> MATTSHQPQDRYKAVWLIFFMLGLGTLLPWNFFMTATQYFTNRLDMSQNVSLVTAELSKDAQASAAPAAPLPERNSLSAIFNNVMTLCAMLPLLLFTYLNSFLHQRIPQSVRILGSLVAILLVFLITAILVKVQLDALPFFVITMIKIVLINSFGAILQGSLFGLAGLFPASYTAAIMSGQGLAGFFASVAMICAIASGSELSESAFGYFITACAVIILTIICYLGLPRLEFYRYYQQLKLEGPTNESHSIKAILKKISVLAFSVCFIFTITIGMFPAVTVEVKSSIAGSSTWERYFIPVSCFLTFNIFDWLGRSLTAVFMWPGKDSRWLPSLVLARLVFVPLLLLCNIKPRRYLTVVFEHDAWFIFFMAAFAFSNGYL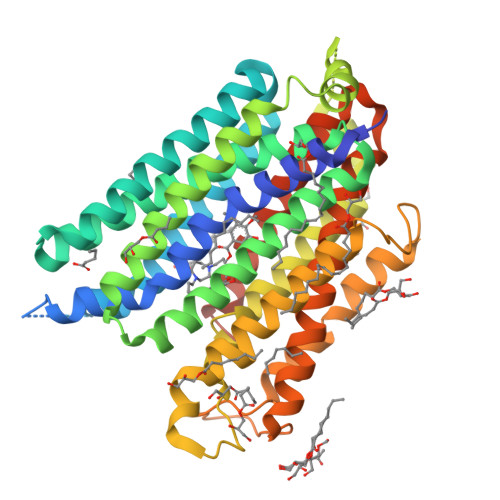ASLCMCFGPKKVKPAEAETAGAIMAFFLCLGLALGAVFSFLFRAIVGTELLQVDTNSLEVLFQ>AQSVDIHKDQIIFSEGDAGDCAYIIEKGRVLIYLTKDKEEIPLTILGEGEIFGEMALIDNQNRSASVRALEDVRLAIVTKQQVLERVSTADKVVQLLMRVLLKRLRRKNIGGPGGSRISEVEFDNSGAGDDGTQSALDQIKLENQIFQAFQNKEFELFYQPIVNLKNKTITGCEALLRWNSPQHGLVSPNLFIDIIENSSMVIPIGHWIINQALKDLRTIQDQLRLNKKERMADDFMMSINISGRQFTHSDFVNNLEDLREKHDLHTQNIKLEMTERIMMDGAIAIDALNQCRSLGYAISI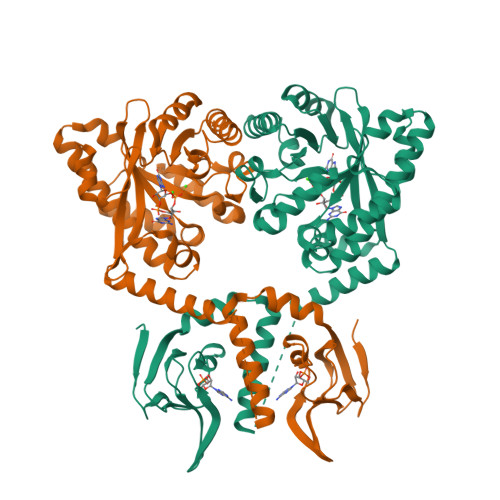DDFGTGFSGLQYLTQMPISFLKIDRSFVMKILSDPKSKAVVSSIIHLAHAMDIEVIAEGIEHHEEALVLETLGARFGQGYLFSKPVDLGRFLKLIKL[2x]> LRHRVLPSSLPNRLFSVDNRETTRFWPPPLQKEEDERRGAFVESCLQPSGKASLLQPPQCLPRAPSHLAKLMEEEERLRLYRHLKKEERDAATLNKFGIWAGEPIADTPAAKMQPLVARTCRQTMRHLQQIEIERLDKQRNFQVPLFGPGDLMEVKYELSRSQQTFATFQGYCVEVRKK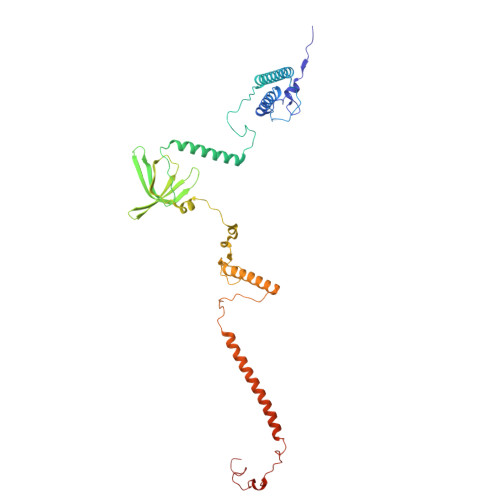RLNSSFVLRNSYEGIGVEQRIPLYSPRIISLKVVSSCASPTQDFLLERHKPLTRDYRYKWKYNFRGRWSRRIGKHKPGIRSVEKKIRQRIVRIRKRYMGQRIEAGLPPYVWGGPYPQYGRKRSLFIRGEMYRRMLIYSFDERRRRAEKLRKRRQAVKWGVFKLRQPSVPPALTALPTYHPLYPGNLPKR>KN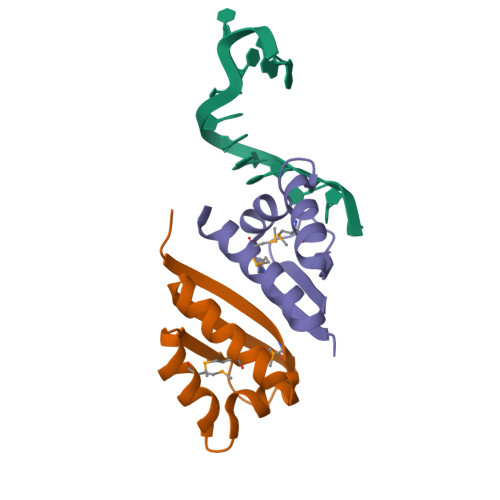VTLTIRLLMHGKEVGSIIGKKGESVKKMREESGARINISEGNCPERIITLAGPTNAIFKAFAMIIDKLEED[4x]> GAMGSGTARPGRSKVFNPYTEFPEFSRRLLKDLEKMFK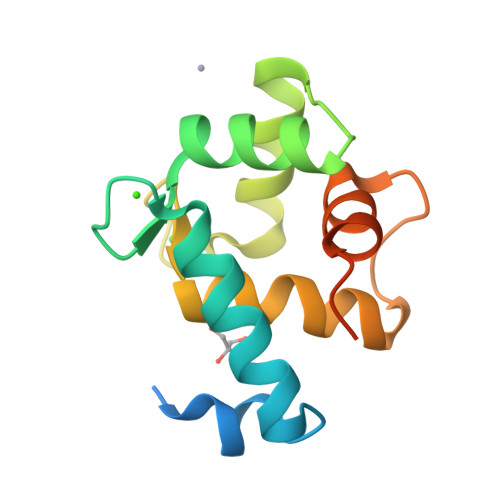TYDAGRDGFIDLMELKLMMEKLGAPQTHLGLKSMIKEVDEDFDGKLSFREFLLIFHKAAAGELQEDSGLLALAKFSEIDVALEGVRGAKNFF> MPSLANGLRCPDALITRTLNPLLNGPKFAVIYCGNHQYKVAVGDVIAVQRLRVEIGSHIALKKVLMVGGPRFT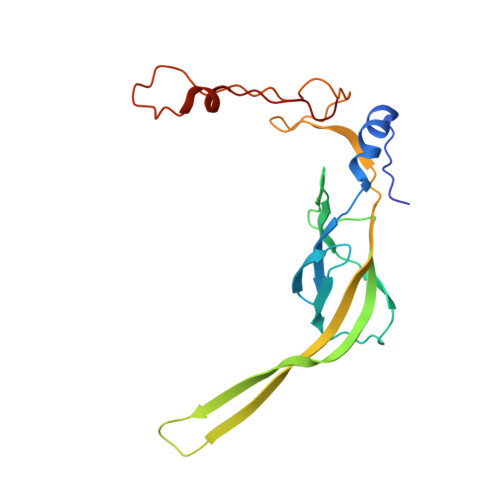AIGRPLLEGVRVTAQVEEQKRMRNVVSLFATPGRRHVRWVDAPHAATIIRICEIFYSPNVVGELDKYKGELLETFTPGQHTNPVYPVDDGYDVFRKKDKEAMENATTFLDLLGGV2'-AMINO-2'-DEOXYADENOSINE | C10 H14 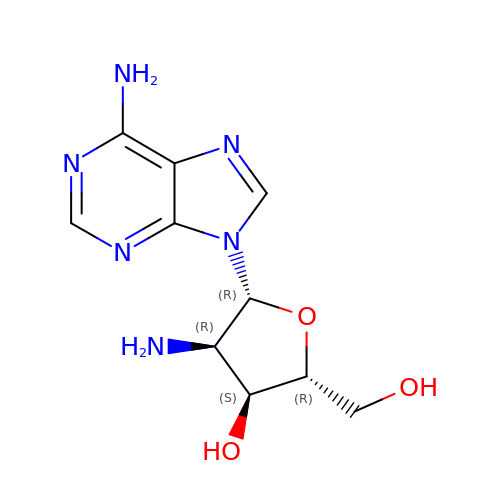N6 O3 | CQKMBZHLOYVGHW-QYYRPYCUSA-N>[2x]MSLGTEEYRIGEIFLAATEENKPQVFANAE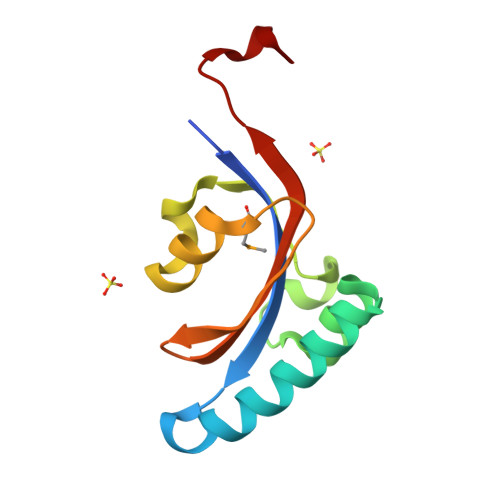KIVEQLKQGGSFVAYARQYSEASTAAVGGDLGWIRLAQLPTELATTAASMGPGQLAGPVEIRGGFSILYLIDKREGHHHHHH> MVNDNAPVFDPYLPRNLSVVEEEANAFVGQVRATDPDAGINGQVHYSLGNFNNLFRITSNGSIYTAVKLNREARDHYELVVVATDGAVHPRHSTLTLYIKVLDIDDNSPVFTNSTYTVVVEENLPAGTSFLQIEAKDVDLGANVSYRIRSPEVKHLFALHPFTGELSLLRSLDYEAFPDQEASITFLAEAFDIYGT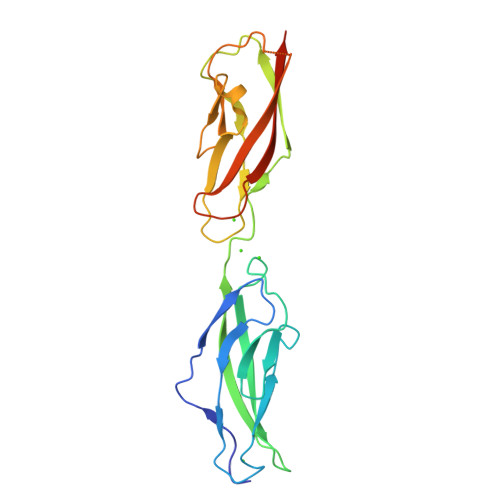MPPGIATVTVIVKDLEHHHHHH> MAGTALKRLMAEYKQLTLNPPEGIVAGPMNEENFFEWEALIMGPEDTXFEFGVFPAILSFPLDYPL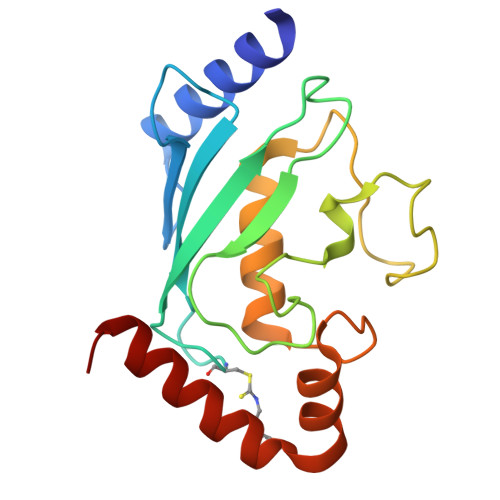SPPKMRFTSEMFHPNIYPDGRVSISILHAPGDDPMGYESSAERWSPVQSVEKILLSVVSMLAEPNDESGANVDASKMWRDDREQFYKIAKQIVQKSLGL> MAELACFCYPHLENDSYKFIPFNNLAIKAMLTAKVDKKDMDKFYDSIIYGIAPPPQFKKRYNTNDNSRGMNFETIMFTKVAMLICEALNSLKVTQANVSNV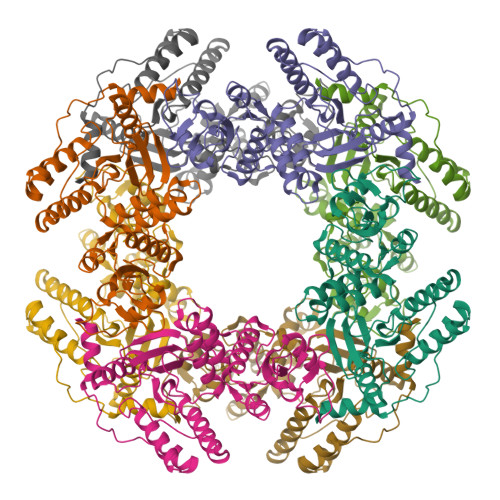LSRVVSIRHLENLVIRKENPQDILFHSKDLLLKSTLIAIGQSKEIETTITAEGGEIVFQNAAFTMWKLTYLEHQLMPILDQNFIEYKVTLNEDKPISDVHVKELVAELRWQYNKFAVITHGKGHYRIVKYSSVANHADRVYATFKSNVKTGVNNDFNLLDQRIIWQNWYAFTSSMKQGNTLDVCKRLLFQKMKPEKNPFKGLSTDRKMDEVS4-[12-[(1-chloranyl-5,6,7-trimethyl-pyrrolo[3,4-d]pyridazin-3-ium-3-yl)methyl]-10,11-dimethyl-3,4,6,7,11-pentazatricyclo[7.3.0.0^{2,6}]dodeca-1(12),2,4,7,9-pentaen-5-yl]-1,2,5-trimethyl-pyrrole-3-carbaldehyde 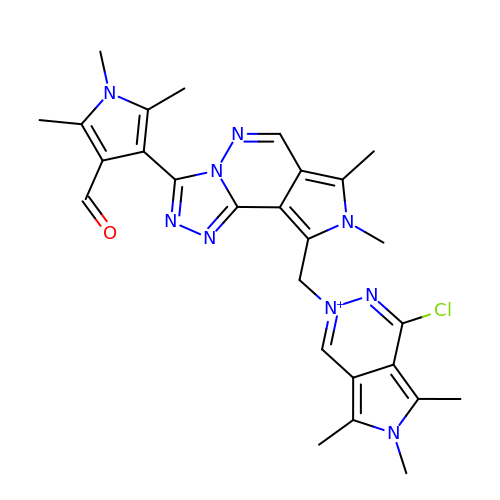| C27 H29 Cl N9 O | NGGFPHTYSIHBDE-UHFFFAOYSA-N>MTSLRDLIPKHKFDNSTIDQLCKLIDNEIEPIIFDLLKWLQDYNWPIAKDILPVVVLHQ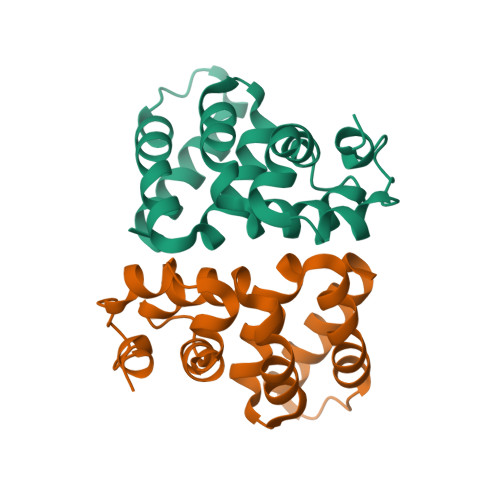SIAMPHILTILQGNDIMWKYWVIKLMIPYLIYPNKQLVKSELERLSSLEIINEDIREIVNLSKDYLHFYYPDKHN[2x]> DLLSCLTFNGVRNHTVFSADSDSDFNRFLHLSIQNPLFQNSLISKPSAIILPGSKEELSNTIRCIRKGSWTIRLRSGGHSYEGLSYTSDTPFILIDLMNLNRVSIDLES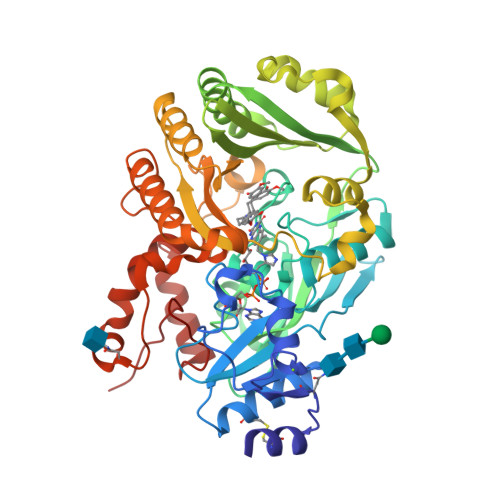ETAWVESGSTLGELYYAITESSSKLGFTAGWAPTVGTGGHISGGGFGMMSRKYGLAADNVVDAILIDANGAILDRQAMGEDVFWAIRGGGGGVWGAIYAWKIKLLPVPEKVTVFRVTKNVAIDEATSLLHKWQFVAEELEEDFTLSVLGGADEKQVWLTMLGFHFGLKTVAKSTFDLLFPELGLVEEDYLEMSWGESFAYLAGLETVSQLNNRFLKFDERAFKTKVDLTKEPLPSKAFYGLLERLSKEPNGFIALNGFGGQMSKISSDFTPFPHRSGTRLMVEYIVAWNQSEQKKKTEFLDWLEKVYEFMKPFVSKNPRLGYVNHIDLDLGGIDWGNKTVVNNAIEISRSWGESYFLSNYERLIRAKTLIDPNNVFNHPQSIPPMANF>[2x]MGVGGDPAVALPHRRFEYKYSFKGPHLVQSDGTVPFWAHAGNAIPSSDQIRVAPSLKSQRGSVWTKTKAAFENWEVEVTFRVTGRGRIGADGLAIWYAENQGLEGPVFGSADLWNGVGIFFDSFDNDGKKNNPAIVIIGNNGQIHYDHQNDGASQALASCQRDFRNKPYPVRAKITY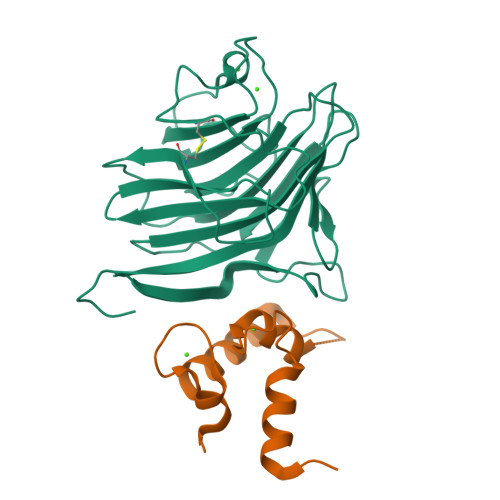YQNTLTVMINNGFTPDKNDYEFCAKVENMIIPAQGHFGISAATGGLADDHDVLSFLTFQLTEPGKEPPTP;>GSHMGVINKPEAEMSPQELQLHYFKMHDYDGNNLLDGLELSTAITHVHKEEGSEQAPLMSEDELINIIDGVLRDDDKNNDGYIDYAEFAKSLQ[2x]> MNYCFAGKTSSISDLKEVPRKNITLIRGLGHGAFGEVYEGQVSGMPNDPSPLQVAVKTLPEVCSEQDELDFLMEALIISKFNHQNIVRCIGVSL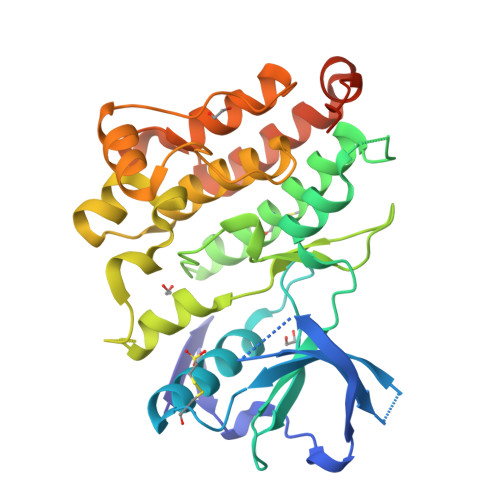QSLPRFILLELMAGGDLKSFLRETRPRPSQPSSLAMLDLLHVARDIACGCQYLEENHFIHRDIAARNCLLTCPGPGRVAKIGDFGMARDIYRASYYRKGGCAMLPVKWMPPEAFMEGIFTSKTDTWSFGVLLWEIFSLGYMPYPSKSNQEVLEFVTSGGRMDPPKNCPGPVYRIMTQCWQHQPEDRPNFAIILERIEYCTQDPDVINTALPIEYGPLVEEEEKLEHHHHHH> GSAHGPSAMVFTVIQGSGEPTDTVLRATTLSCAYTAEGTHPAPRAACDALN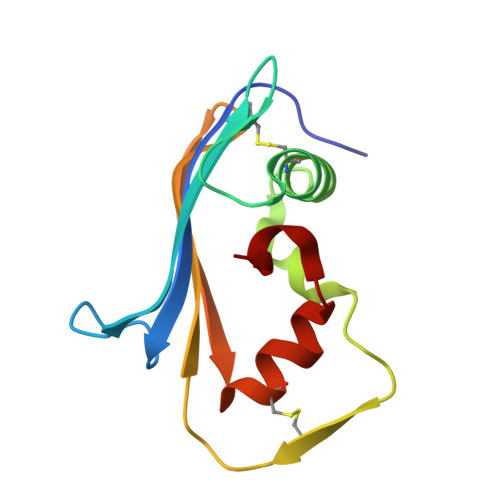ATDGELNRLLAAPDPSLVCPMYFDPVTVTADGVLNGRRVAWKHTFSNTCVMSANLNSNPVYAF> QEALTTQYSQSELLKNWALSHCLALVYKDDVVKNDARATASAYLEYGKQSVEIYHEIDEIAKK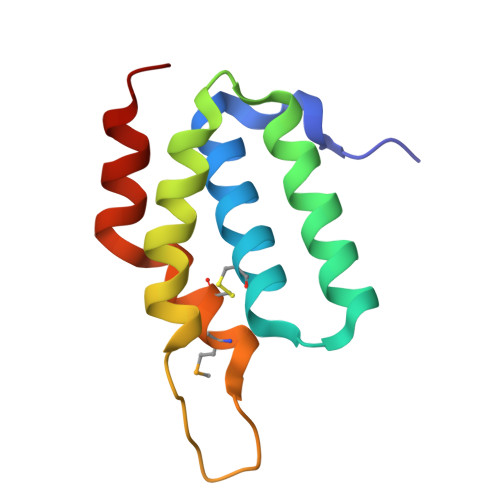YSGLKYNGSISSDFNTMKCIDFIHDRELNELIKRRVEK3-(5-AMINO-7-HYDROXY-[1,2,3]TRIAZOLO[4,5-D]PYRIMIDIN-2-YL)-BENZOIC 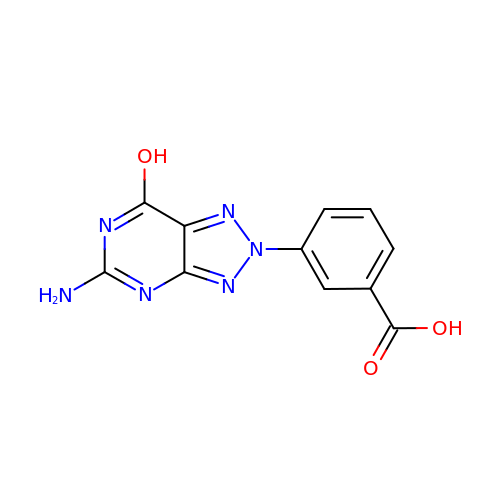ACID | C11 H8 N6 O3 | KNLLRZNGRRRPEW-UHFFFAOYSA-N> MHHHHHHGMEEVTIKANLI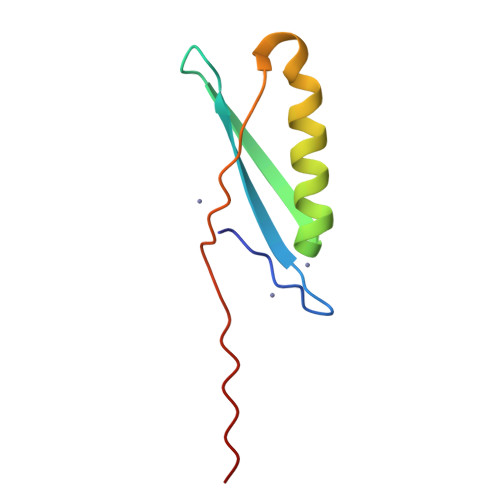FANGSTQTAEFKGTFEKATSEAYAYADTLKKDNGEWTVDVVPKAYTLNIKFAG>UGGAAGAAAUCGAAGAAGAUGAAGAACGCGAAGAAC[2x];>AUCUUCUUCGAUUUCUUCCAGUUCUUCGCGUUCUUC[2x]

Recently, RNA-catalyzed rolling circle synthesis (RCS) on small circular RNA (scRNA) templates has been demonstrated. To gain deeper insight into the RCS process and the strong inhibition observed upon full-length circle synthesis, we used cryo-EM to study the structure of putative RCS replication products formed by complexing the full-length scRNA and nascent complementary RNA (cmpRNA). To our surprise, cryo-EM revealed not one by a diverse variety of distinct structural species identified as monomers, dimers, and multimers of the scRNA–cmpRNA complex. We find that scRNAs and cmpRNAs of 36 nt in length can form an unanticipated diversity of structures with different stoichiometries, including a fully annealed dimer (comprising two scRNAs and two cmpRNAs) and multimers hereof.

Class 2 showed density similar to two parallel RNA helices, one long and one shorter. The low-resolution cryo-EM maps of classes 1 and 2 are consistent with partly hybridized scRNA and cmpRNA. The low-resolution density map for class 2 was consistent with a model composed of two scRNAs and two cmpRNAs, where the second cmpRNA had only partly hybridized. Based on the dimer model derived from class 3, we propose a model for class 2, where one cmpRNA is fully hybridized and the other cmpRNA is partly hybridized. Based on the position of the major grooves in the class 2 map, we can deduce that it is the 3′-end of one of the cmpRNAs that does not hybridize. Furthermore, class 2 has the potential to form via two different pathways where either the 5′- or 3′-end does not anneal. Interestingly, class 2 might represent a trapped state of the rolling mechanism, where only one of the unpaired ends has hybridized by the rolling mechanism (class 2). Classes 1 and 2 were poorly resolved but resemble RCS structures as predicted by our MD simulation and may represent intermediates trapped on the way to dimer formation.>[2x]HDRLGESKEDDTLRRFRYLLGLTDLFRHFIETNPNPKIREIMKEIDRQNEEEARQRKRGGRQGGATSERRRRTEAEEDAELLKDEKDGGSAETVFRESPPFIQGTMRDYQIAGLNWLISLHENGISGILADEMGLGKTLQTIA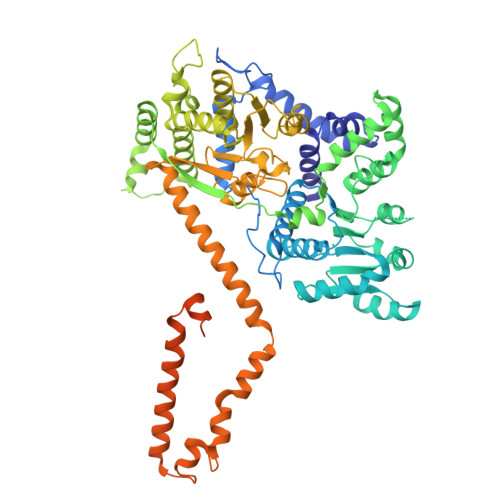FLGYLRHIMGITGPHLVTVPKSTLDNWKREFEKWTPEVNVLVLQGAKEERHQLINDRLVDENFDVCITSYEMILREKAHLKKFAWEYIIIDEAHRIKNEESSLAQVIRMFNSRNRLLITGTPLQNNLHELWALLNFLLPDVFGDSEAFDQWFSGQDRDQDTVVQQLHRVLRPFLLRRVKSDVEKSLLPKKEINVYIGMSEMQVKWYQKILEKDIDAVNGAGGKRESKTRLLNIVMQLRKCCNHPYLFEGAEPGPPYTTDEHLIYNAGKMVVLDKLLKRIQKQGSRVLIFSQMSRLLDILEDYCVFRGYKYCRIDGSTAHEDRIAAIDEYNKPGSDKFIFLLTTRAGGLGINLTTADIVILYDSDWNPQADLQAMDRAHRIGQTKQVVVYRFVTDNAIEEKVLERAAQKLRLDQLVIQQGRAQVAAKAAANKDELLSMIQHGAEKVFQTKGAFGTMAEKGSQLDDDDIDAILQAGETRTKELNARYEKLGIDDLQKFTSESAYEWNGEDFAARKKDIGINWINPAKRERKEQIYSIDKYYKQTFNAGGRAAEAKPKAPRAPKQVPVHDYQFYPPRLRELQD4-nitrophenyl 2-amino-2-deoxy-beta-D-glucopyranoside | C12 H16 N2 O7 | 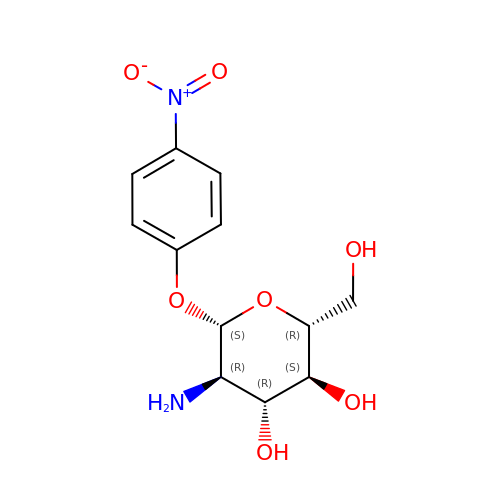ZRNBGANFPXCMFT-LZQZFOIKSA-N> GEAD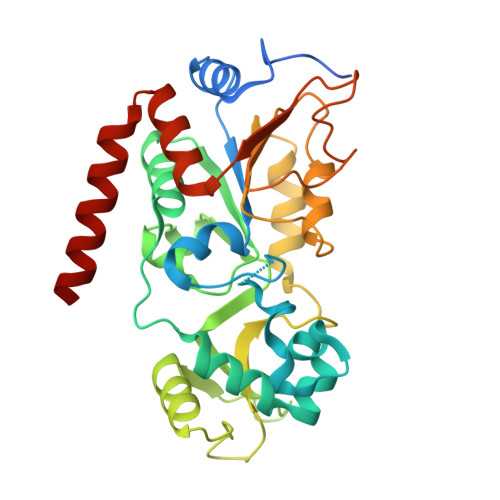MDFLRNLFSQTLSLGSQKERLLDELTLEGVARYMQSERCRRVICLVGAGISTSAGIPDFRSPSTGLYDNLEKYHLPYPEAIFEISYFKKHPEPFFALAKELYPGQFKPTICHYFMRLLKDKGLLLRCYTQNIDTLERIAGLEQEDLVEAHGTFYTSHCVSASCRHEYPLSWMKEKIFSEVTPKCEDCQSLVKPDIVFFGESLPARFFSCMQSDFLKVDLLLVMGTSLQVQPFASLISKAPLSTPRLLINKEKAGQSDPFLGMIMGLGGGMDFDSKKAYRDVAWLGECDQGCLALAELLGWKKELEDLVRREHASIDAQS> ENLKLGFLVKQPEEPWFQTEWKFADKAGKDLGFEVIKIAVPDGEKTLNAIDSLAASGAKGFVICTPDPKLGSAIVAKARGYDMKVIAVDDQFVNAKGKPMDTVPLVMLAATKIGERQGQELYKEMQKRGWDVKESAVMAITANELDTARRRTTGSMDAL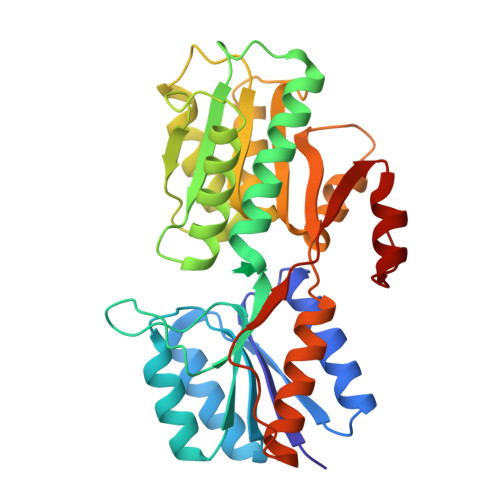KAAGFPEKQIYQVPTKSNDIPGAFDAANSMLVQHPEVKHWLIVGMNDSTVLGGVRATEGQGFKAADIIGIGINGVDAVSELSKAQATGFYGSLLPSPDVHGYKSSEMLYNWVAKDVEPPKFTEVTDVVLITRDNFKEELEKKGLGGK> MIIRRYLVKQVVSTSLVVIALLTLIMMGGRLIKYFGVAAQGRLDAGVLFSIIGYRMPEFLTLILPLGFFIGLMLVFGRLYVDHEMAVLNGSGISRIRLGQLLIPLALVFLVIQGILMLWMTPWGLRQFDQLSSSQAVRTGFDLVRPKEFISSGPYTIYAGDLSEDRKNLKDIFFYQRAQKEGKPDVMILAKEATRVVMENETANVVDLIQGRRYEIYPGKAKYSQAEFQRYRLRLENDKSATFETDKVEALPSSKLWNKWNDPVIASEMGWRVFGPFTIVIALMMAVALCEVSPRQGRYYRLIPAIFIFASLIVLL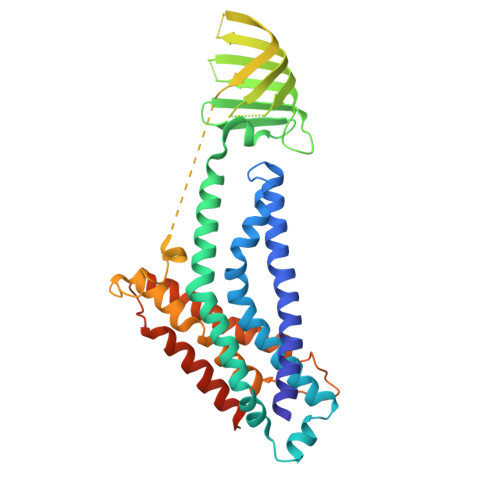IAIRTRISRDELGVWAYPAALAVYGIAAALFSRKQKLAPKIKKQIKRVRA CARD9 functions in myeloid cells during innate immune responses to activate NF-κB and p38 MAPK. CARD9 and CARD11 share an N-terminal domain architecture comprising an N-terminal CARD followed by ~300 residues with high coiled-coil propensity, referred to as the coiled-coil domain. Upon activation, both CARD9 and CARD11 recruit the same downstream binding partner, B-cell lymphoma/leukemia 10 (Bcl10), which interacts through its own CARD with the CARD of CARD9 or CARD11, a CARD–CARD interaction critical for subsequent signal propagation and NF-κB activation. The CARDs of CARD9 or CARD11 are thought to form a nucleating helical template that promotes polymerization of Bcl10 via the Bcl10 CARD, which, along with other domains of activated CARD9/11, then recruits downstream factors, including MALT1, cIAPs, TRAF6, and the LUBAC complex that mediate subsequent ubiquitination of multiple members of the complex, including both linear and K63-linked poly-ubiquitination of Bcl1013–16.

We found that CARD92−152/I107E spontaneously formed filaments after a short incubation at elevated temperatures, which are readily visible by negative-stain electron microscopy (NS-EM). With the CARD92−152/I107E construct, however, we found that the filaments now remained predominantly singular when frozen shortly after inducing filament formation. With this sample, we were able to generate a 4.0-Å reconstruction of the CARD9 CARD filament. The coiled-coil domain is disordered relative to the CARD core, such that the reconstruction contains only CARD residues 8–95. The CARD adopts the canonical helical architecture of a death domain, with helical symmetry of a 5.11 Å rise and 101.6° left-handed rotation, consistent with a growing body of literature demonstrating a narrow range of parameters adopted by helical assemblies of CARDs (4.85–5.13 Å rise and 100.2°−101.6° left-handed rotation) including that of Bcl1036,38–41. As is typical of this architecture, the CARD utilizes three CARD-CARD interfaces, known as the Type I, Type II, and Type III interfaces, corresponding to the 3-, 4-, and 1-start helical symmetries, respectively. As detailed in Fig. 6c, interactions within the interfaces are predominantly electrostatic in nature, consistent with our previous observation that increasing salt concentration can inhibit assembly. As monitored by A350 and NS-EM, mutation of residues in the Type I (E15R, R35E, D66R), Type II (R29D), or Type III (D43R, K58D) interfaces completely blocked filament formation when tested up to a 1 mM concentration. The exception is the flexible α3-α4 loop, which adopts a ‘closed’’ conformation in the NMR structure, but an “open” conformation in the filament, stabilized by interactions across the Type III interface.

>GSDYENDDECWSVLEGFRVTLTSVIDPSRITPYLRQCKVLNPDDEEQVLSDPNLVIRKRKVGVLLDILQRTGHKGYVAFLESLELYYPQLYKKVTGKEPARVFSMIEDASGESGLTQLLMTEVMKLQKKVQDLTALLSSKDDFIKELRVKDS[10x]> MTPLGPASSLPQSFLLKCLEQVRKIQGDGAALQEKLCATYKLCHPEELVLLGHSLGIPWAPLSSCPSQALQLAGCLSQLHSGLFLYQGLLQALEGISPELGPTLDTLQLDVADFATTIWQQMEE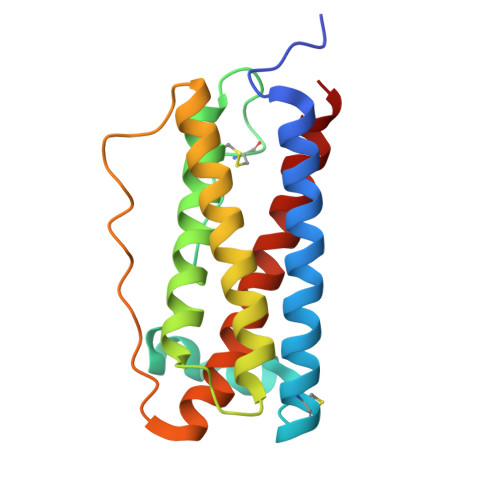LGMAPALQPTQGAMPAFASAFQRRAGGVLVASHLQSFLEVSYRVLRHLAQP> AFTDV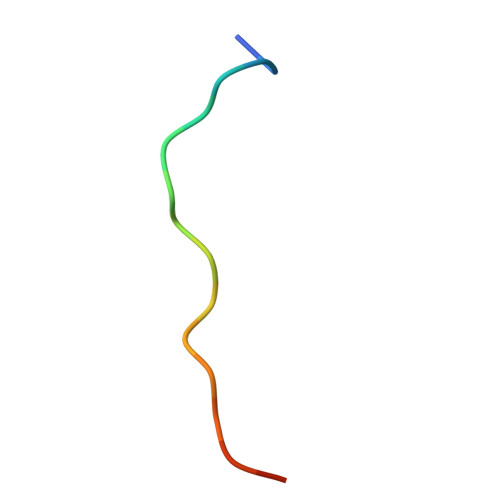PALNYPATPPPH> GAMAMTTDEGAKNNEES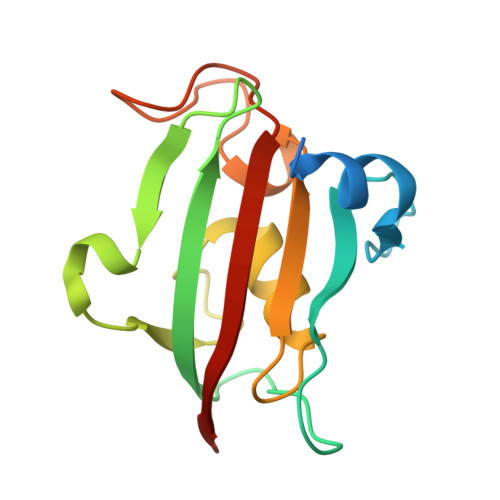PTATVAEQGEDITSKKDRGVLKIVKRVGNGEETPMIGDKVYVHYKGKLSNGKKFDSSHDRNEPFVFSLGKGQVIKAWDIGVATMKKGEICHLLCKPEYAYGSAGSLPKIPSNATLFFEIELLDFKGE> MGPGSDKDCEMKRTTLDSPLGKLELSGCEQGLHEIIFLGKGTSAADAVEVPAPAAVLGGPEPLMQA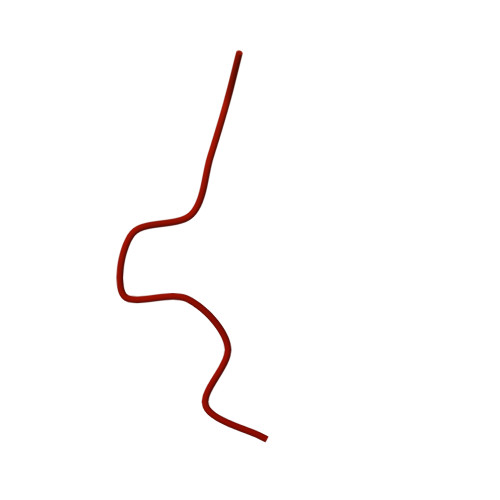TAWLNAYFHQPEAIEEFPVPALHHPVFQQESFTRQVLWKLLKVVKFGEVISYSHLAALAGNPAATAAVKTALSGNPVPILIPCHRVVQGDLDVGGYEGGLAVKEWLLAHEGHRLGKRGGGSGGGSPEKRLTVGSLRR> GMDNWQDITDDR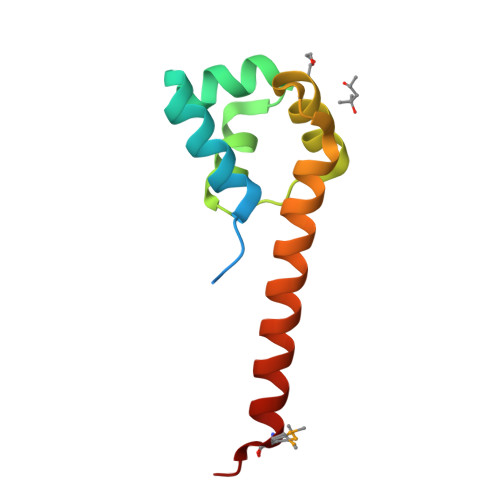LVRPIHPGEVIADILDDLDINTANFAEILGVSNQTIQEVINGQRSITVDIAIRLGKALGNGPRLWLNLQQKVDLWYALQSHKEEYEQVMTLV2'-DEOXYADENOSINE 5'-O-(1-THIOTRIPHOSPHATE) | C10 H16 N5 O11 P3 S | 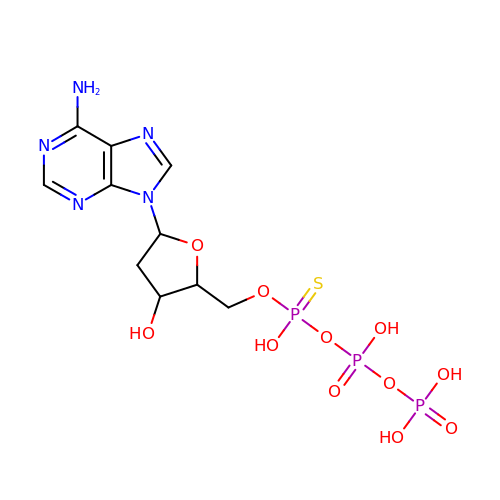CCPIKNHZOWQALM-XZPDCLKESA-N>AACLPDIIFDEPSQGPEKNEAISMLTERLSSIINAAGGDIGIAVIHVETG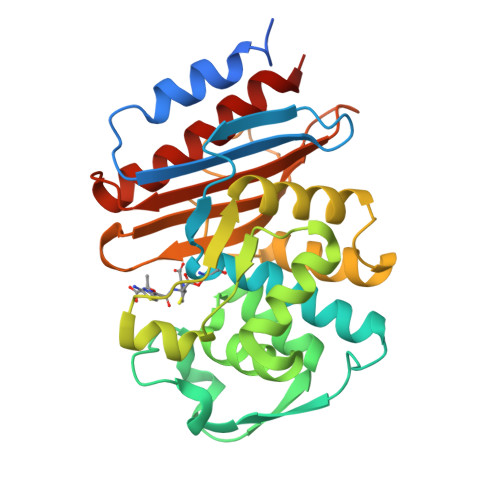HTTAIQGTTQLPLYSVFKLPLAIAVLKEIEENRLQLDRKVRVTPADVAPGWTANAAMWRRPIDRTVAQLIEVSIIRSDNTSSDKLLQLVGGPAAVTHRMRALGFPNIEIVSTVREFSENRTRPNTGSAEDLARLLVQLQKGELLQPQHSALLLGFMHRATTGTERLRGSLPVGTPVADKTGTGDAGVVTNDVGIITLPKGQGHLAIAVLISGSKLSPAAQEKLIAEIARAAYDAHVSRAE[2x]>[2x]MKIYQKRLEYYTDSRDYDNLRSLSPLSDSSVNKSPEEHKQDAESEKNLKNINPDYRFWIKVEG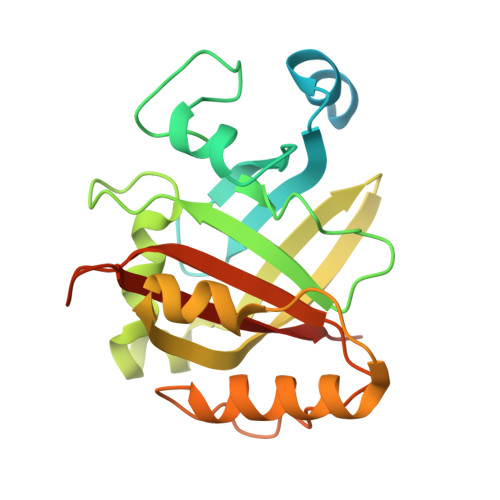TNIDFPVVQGKDNDFYLHHNFNKEKSFSGSIFVDSENNLNDDSNIVVYGHNMRNDTMFAQIKHFKNENFFNANKYVTLYREGKKSTFEIFSVYQENAKDLESEIKTKFSNKEDYEKYLKEQESKSLFKRDGIDLNSNDRILTLITCGYDFVNARIVVVAKEIDLEHHHHHH N-[(1S)-2-[(4-cyano-1-methylpiperidin-4-yl)amino]-1-(cyclohexylmethyl)-2-oxoethyl]morpholine-4-carboxamide 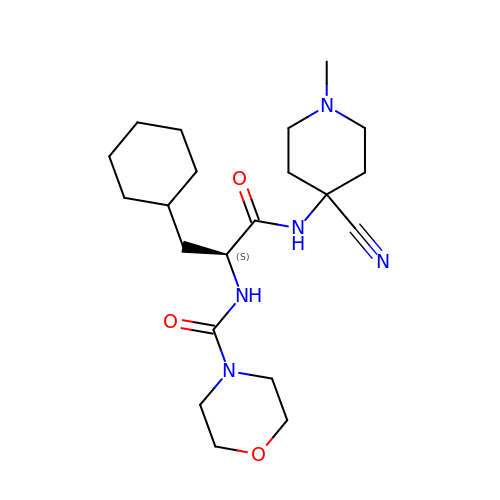| C21 H35 N5 O3 | IRSOCWQJNYLTDD-SFHVURJKSA-N> MSSTVIAFGDPKAQKKWSSELAVDIRKKSYFESRFIGTSENAVIQRKTEVESDAGDRVSFDLSVRLRGQPTFGDDRVEGKEENLKFYTDEVIIDQVRHSVSAGGRMSRKRTAHDLRKTGRDRLGDYFYQLTDELFFMYLSGARGINKDFILPTSFTGYAKNPFNTPDAAHLLYGGVATSKASLANTDTMSRVVIERANVQATMMQAQDPETANMVPVSVEGEDRYVCVMSPFQEHSLRTSDAAGWLEIQKAAAAAEGRNNPIFKGGLGMIGNTVLH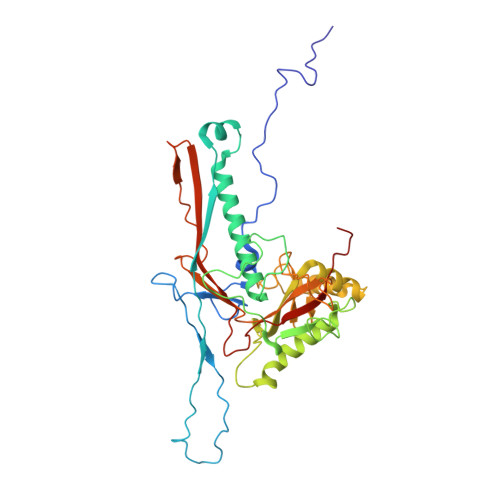SHRNVVRFSDYGAGSDQPAARALFMGRQAAVVAYGTKGGLRYDWQEETKDYGNEPTVASGFIAGIKKTRFNDRDFGVISIDTYAKDPNPNNPA> QSACTLQSETHPPLTWQKCSSGGTCTQQTGSVVIDANWRWTHATNSSTNCYDGNTWSSTLCPDNETCAKNCCLDGAAYASTYGVTTSGNSLSIGFVTQSAQKNVGARLYLMASDTTYQEFTLLGNEFSFDVDVSQLPCGLNGALYFVSMDADGGVSKYPTNTAGAKYGTGYCDSQCPRDLKFINGQANVEGWEPSSNNANTGIGGHGSC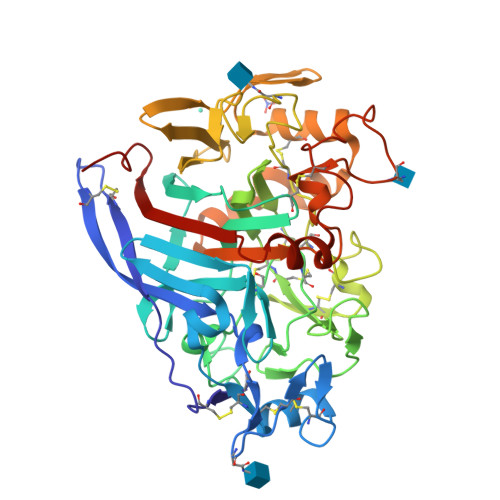CSEMDIWEANSISEALTPHPCTTVGQEICEGDGCGGTYSDNRYGGTCDPDGCDWNPYRLGNTSFYGPGSSFTLDTTKKLTVVTQFETSGAINRYYVQNGVTFQQPNAELGSYSGNELNDDYCTAEEAEFGGSSFSDKGGLTQFKKATSGGMVLVMSLWDDYYANMLWLDSTYPTNETSSTPGAVRGSCSTSSGVPAQVESQSPNAKVTFSNIKFGPIGSTGNP>GSHMVPISFVFNRFPRMVRDLAKKMNKEVNFIMRGEDTELDRTFVEEIGEPLLHLLRNAIDHGIEPKEERIAKGKPPIGTLILSARHEGNNVVIEVEDDGRGIDKEKIIRKAIEKGLIDESKAATLSDQEILNFLFVPGFSTKEKVSEVSGRGVGMD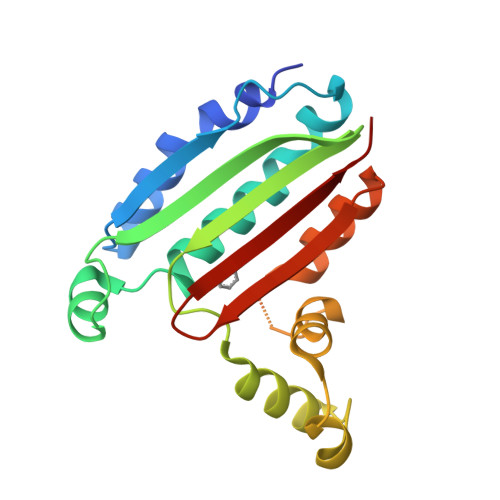VVKNVVESLNGSISIESEKDKGTKVTIRLPLT[2x]3-(pyridin-2-yloxy)aniline | C11 H10 N2 O 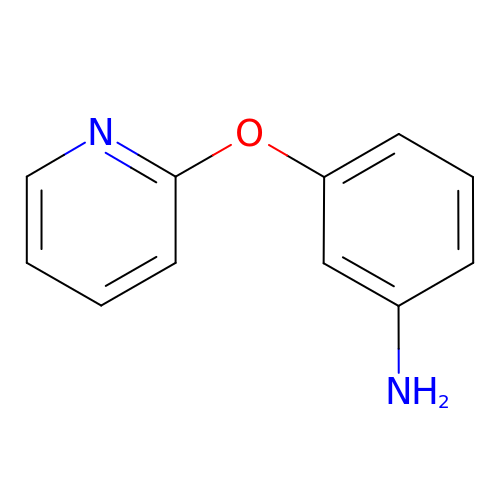| CLQMOPKXIBQKKG-UHFFFAOYSA-N>MFSKLAHLQRFAVLSRGVHSSVASATSVATKKTVQGPPTSDDIFEREYKYGAHNYHPLPVALERGKGIYLWDVEGRKYFDFLSSYSAVNQGHCHPKIVNALKSQVDKLTLTSRAFYNNVLGEYEEYITKLFNYHKVLPMNTGVEAGETACKLARKWGYTVKGIQKYKAKIVFAAGNFWGRTLSAISSSTDPTSYDGFGPFMPGFDIIPYNDLPALERALQDPNVAAFMVEPIQGEAGVVVPDPGYLMGVRELCTRHQVLFIADEIQTGLARTGRWLAVDYENVRPDIVLLGKALSGGLYPVSAVLCDDDIMLTIKPGEHGSTYGGNPLGCRVAIAALEVLEEENLAENADKLG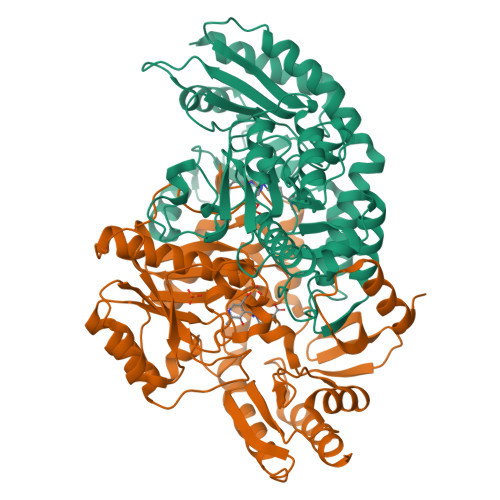IILRNELMKLPSDVVTAVRGKGLLNAIVIKETKDWDAWKVCLRLRDNGLLAKPTHGDIIRFAPPLVIKEDELRESIEIINKTILSF[3x]>[4x]MDSLQKQDLRRPKIHGAVQASPYQPPTLASLQRLLWVRQAATLNHIDEVWPSLFLGDAYAARDKSKLIQLGITHVVNAA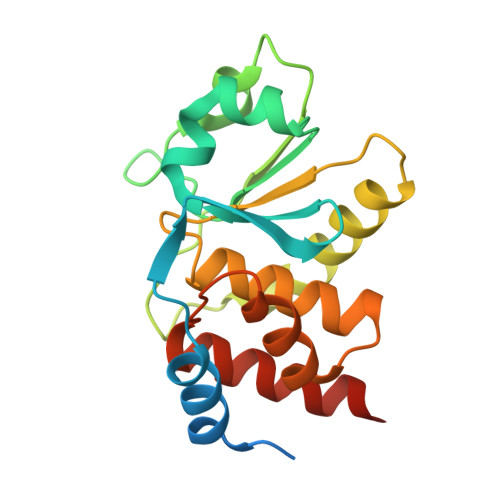AGKFQVDTGAKFYRGMSLEYYGIEADDNPFFDLSVYFLPVARYIRAALSVPQGRVLVHCAMGVSRSATLVLAFLMICENMTLVEAIQTVQAHRNICPNSGFLRQLQVLDNRLGRETGRF>SLKLAKNVEIEIRTKIHPTESEDKVLKAIRNIFPDAEIEISEEGEVYGRAYSLDRFRELLRKQRILDTARSEILKGRNGKEVTIYLNKQTATVSRINFCDENAVLSPIKVTFRLNNIP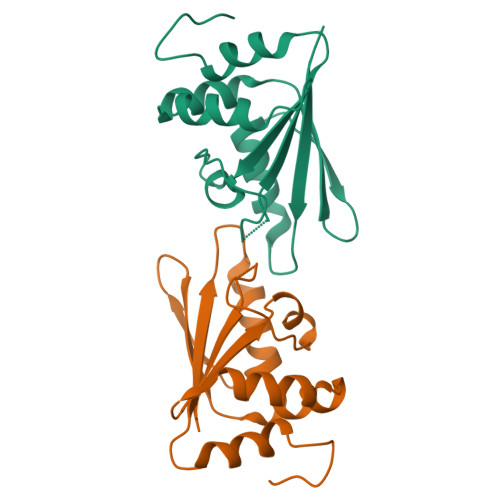FSRFLDYIAPETKDGRPVKEIDKL[2x]> MTSKGPEEEHPSVTLFRQYLRIRTVQPKPDYGAAVAFFEETARQLGLGCQKVEVAPGYVVTVLTWPGTNPTLSSILLNSHTDVVPVFKEHWSHDPFEAFKDSEGYIYARGAQDMKCVSIQYLEAVRRLKVEGHRFPRTIHMTFVPDEEVGGHQGMELF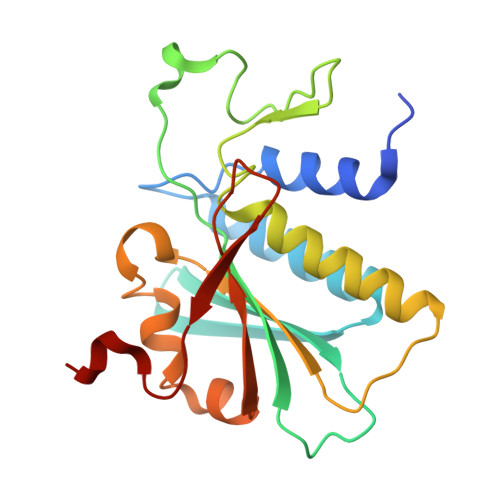VQRPEFHALRAGFALDEGIANPTDAFTVFYSERSPWWVRV>[2x]AALPDQSFLWNVFQRVDKDRSGVISDTELQQALSNGTWTPFNPVTVRSIIS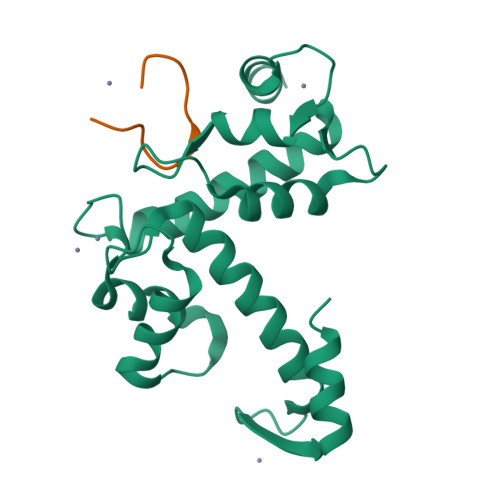MFDRENKAGVNFSEFTGVWKYITDWQNVFRTYDRDNSGMIDKNELKQALSGFGYRLSDQFHDILIRKFDRQGRGQIAFDDFIQGCIVLQRLTDIFRRYDTDQDGWIQVSYEQYLSMVFSIV;>[2x]NPPPPGFIMHGN Here we report the biochemical and structural characterization of B. anthracis (Ames) alanine racemase (AlrBax), an essential enzyme in prokaryotes and a target for antimicrobial drug development. The enzyme utilizes a pyridoxal 5'-phosphate (PLP) cofactor to catalyze the racemization of L-alanine to D-alanine, an essential component of the peptidoglycan layer in bacterial cell walls. The lack of alanine racemase function in eukaryotes has made this enzyme an attractive target for antimicrobial drug development. The dal1 gene product (AlrBax) is found on the spores' outermost layer and addition of alanine racemase inhibitors has been shown to promote germination of B. anthracis' spores while endogenous production of D-alanine, mediated by alanine racemase, inhibits germination.

Consistent with other alanine racemases, the tertiary structure of AlrBax is a homodimer formed by head-to-tail-association of two monomers. Residues in the N-terminus (16–245) fold into an eight-stranded α/β barrel, while the C-terminal residues (246–389) and the first 15 N-terminal amino acids are part of a predominantly β-structure. The homodimer displays two active sites, formed by residues from the N-terminus of one monomer and residues from the C-terminus of the other monomer. The PLP cofactor forms a covalent bond to Lys41 and points at the center of the α/β barrel. As previously observed for AlrGst, extra density was present in the active of AlrBax, which we model here as a molecule of acetate. The oxygen atoms from the acetate molecule in our model are within hydrogen bonding distance to the side chain oxygen from Tyr289', the main chain nitrogen from Met317' and, perhaps more importantly, to the side chain nitrogen atom from the catalytic Lys41 residue. One striking difference in the active site involves Asn131, which in other alanine racemases is generally a carbamylated lysine that participates in a hydrogen bond with the residue homologous to Arg138. In AlrBax, however, we note a prominent chloride ion that is located near Arg138 in the active site. As AlrBax lacks the conserved lysine residue necessary for carbamylation it has apparently drafted a chloride ion to fill the same role for this species. Our analyses of both structures suggest that despite differences in space group and crystal lattice, reductive methylation does not significantly alter the structure of alanine racemase from B. anthracis.

>[2x]MEEAPFYRDTWVEVDLDAIYNNVTHIKEFIPSDVEIFAVVKGNAYGHDYVPVAKIALEAGATRLAVAFLDEALVLRRAGITAPILVLGPSPPRDINVAAENDVALTVFQKEWVDEAIKLWDGSSTMKYHINFDSGMGRIGIRERKELKGFLKSLEGAPFLELEGVYTHFATADEVETSYFDKQYNTFLEQLSWLKEFGVDPKFVHTANSAATLRFQGITFNAVRIGIAMYGLSPSVEIRPFLPFKLEPALSLHTKVAHIKQVIKGDGISYNVTYRTKTEEWIATVAIGYADGWLRRLQGFEVLVNGKRVPIVGRVTMDQFMIHLPCEVPLGTKVTLIGRQGDEYISATEVAEYSGTINYEIITTISFRVPRIFIRNGKVVEVINYLNDILEENLYFQ>GS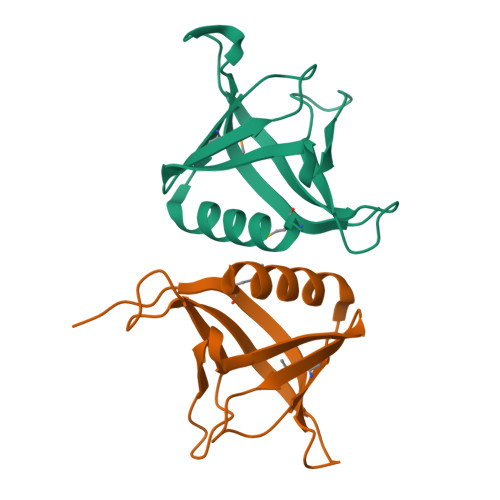MAPPAGGAAAAASDLGSAAVLMAVHAAVRPLGAGPDAEAQLRRLQLSADPERPGRFRLELLGAGPGAVNLEWPLESVSYTIRGPTQHELQPPPGGPGTLSMHFLNPQEAQRWAVLVRGATVEGQNGS[4x]> MARQNLKSTDRAVQQMLDKAKREGIQTVWDRYEAMKPQCGFGETGLCCRHCLQGPCRINPFGDEPKVGICGATAEVIVARGLDRSIAAGAAGHSGHAKHLAHTLKKAVQGKAASYMIKDRTKLHSIAKRLGIPTEGQKDEDIALEVAKAALADFHEKDTPVLWVTTVLPPSRVKVLSAHGLIPAGIDHEIAEIMHRTSMGCDADAQNLLLGGLRCSLADLAGCYMGTDLADILFGTPAPVVTESNLGVLKADAVNVAVHGHNPVLSDIIVSVSKEME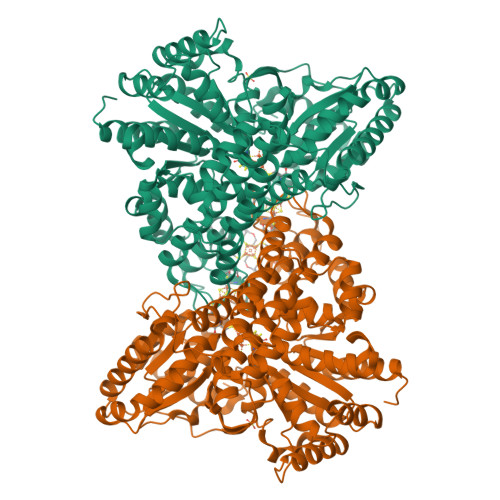NEARAAGATGINVVGICDTGNEVLMRHGIPACTHSVSQEMAMITGALDAMILDYQCIQPSVATIAECTGTTVITTMEMSKITGATHVNFAEEAAVENAKQILRLAIDTFKRRKGKPVEIPNIKTKVVAGFSTEAIINALSKLNANDPLKPLIDNVVNGNIRGVCLFAGCNNVKVPQDQNFTTIARKLLKQNVLVVATGCGAGALMRHGFMDPANVDELCGDGLKAVLTAIGEANGLGGPLPPVLHMGSCVDNSRAVALVAALANRLGVDLDRLPVVASAAEAMHEKAVAIGTWAVTIGLPTHIGVLPPITGSLPVTQILTSSVKDITGGYFIVELDPETAADKLLAAINERRAGLGLPW> MSMAEMLRRDEGLRLKVYWDTEGYPTIGIGHLIMKQPVRDMAQINKVLSKQVGREITGNPGSITMEEATTLFERDLADMQRDIKSHSKVGPVWQAVNRSRQMALENMAFQMGVGGVAKFNTMLTAMLAGDWEKAYKAGRDSLWYQQTKGRASRVTMIILTGNLESYGVELEHHHHHH;> MKKFIFATIFALASCAAQPAMAGYDKDLCEWSMTADQTEVETQIEADIMNIVKRDRPEMKAEVQKQLKSGGVMQYNYVLYCDKNFNNKNIIAEVVGELEHHHHHH

One of the T4 early gene products produced immediately following the genome injection is gp61.3, also known as Spackle. Spackle, along with another T4 gene product Imm, confers the infected host E. coli with resistance against secondary phage infections—a phenomenon known as “superinfection exclusion”. Our results show that T4 Spackle forms a stoichiometric complex with the lysozyme domain of gp5 and potently inhibits its enzymatic activity, whereas Spackle does not appreciably inhibit the cytoplasmic T4 lysozyme (endolysin, gpe) responsible for cell lysis at the final step of the phage lytic cycle. Crystal structure of the Spackle–gp5 complex shows that the binding of Spackle induces an allosteric conformational change in the gp5 lysozyme active site and partially blocks its oligosaccharide-binding cleft.

To that end, we co-crystallized Spackle and gp5 lysozyme and determined the crystal structure of the complex by molecular replacement phasing. Two crystal forms were obtained, in monoclinic and orthorhombic lattice systems, for which the structures were refined to 1.78 and 1.92 Å resolution, respectively. The monoclinic crystal contained two Spackle–gp5 lysozyme complexes in the asymmetric unit, whereas the orthorhombic crystal contained one complex in the asymmetric unit. As expected, the crystal structures show a 1:1 Spackle–gp5 lysozyme complex. In addition, we observed several 4-(2-hydroxyethyl)-1-piperazineethanesulfonic acid (HEPES) molecules bound on the lysozyme surface, including one occupying the oligosaccharide-binding cleft (C-site)20 and another in the peptide-binding groove in the monoclinic crystal structure. The protein structures of the three crystallographically independent complexes were essentially identical to each other, with pairwise backbone room mean square deviations within 0.5 Å. Spackle binds to gp5 lysozyme primarily via three short helices (α1, α4, and α5) located on one side of its flat helical bundle fold. The interface buries a total of 952 Å2 surface area and involves numerous polar contacts. The side chains of a number of basic amino acid residues of gp5 lysozyme, namely Arg181, Arg182, Arg187, and Lys189 from the N-terminal lobe and Arg312, Lys321, and Arg326 from the C-terminal lobe, are involved in intermolecular hydrogen bonds or salt bridges with Spackle. Superposition of Spackle and gp5 lysozyme structures in the complex with their respective unbound state structures shows conformational changes for both proteins upon binding. The partial loss of disulfide linkage may reflect the conformational strain in α1 helix upon lysozyme binding and resulting bond breakage or preferential binding of Spackle in the reduced form during crystallization. These observations suggest that Spackle–gp5 lysozyme interaction is mediated by mutual conformational changes, likely via an induced-fit mechanism.>GPLGSRPWQILSQALGFPNYDQELWWQNTAETLNRVLEQCDYSVHLQYKYLAFYHKYILPSLGPF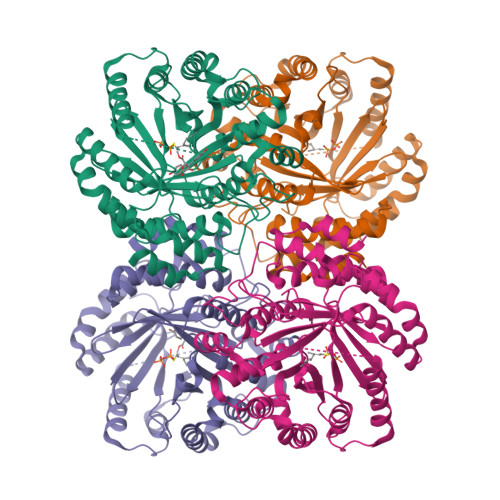RRPGVEPEYISGLSHGGHPLAISVKIDKSKTICRLGLQAIGPLAGTARDPLNSFGDRELLKNLATLLPHVDLRLFDHFNAQVGLDRAQCAVATTKLIKESHNIVCTSLDLKDGEVIPKVYFSTIPKGLVTETPLFDLTFAAIEQMEVYHKDAPLRTALSSLKDFLRPRVPTDASITPPLTGLIGVDCIDPMLSRLKVYLATFRMDLSLIRDYWTLGGLLTDAGTMKGLEMVETLAKTLKLGDEACETLDAERLPFGINYAMKPGTAELAPPQIYFPLLGINDGFIADALVEFFQYMGWEDQANRYKDELKAKFPNVDISQTKNVHRWLGVAYSETKGPSMNIYYDVVAGNV[2x]> CVICDPSVVLALKSLEKDYLPGHLDAKHHKAMMERVENAVKDFQELSLNEDAYMGVVDEATLQKGSWSLLKDLKRITDSDVKGDLFVKELFWMLHLQKETFATYVARFQKEAYCPNKCGVMLQTLIWCKNCKKEVHACRKSYDCGERNVEVPQMEDMILDCELNWHQASEGL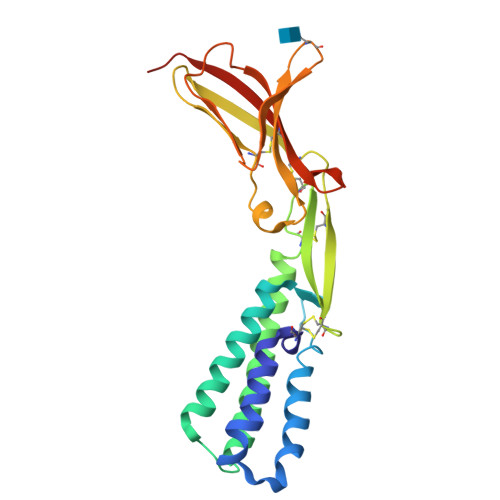TDYSFYRVWGNNTETLVSKGKEATLTKPMVGPEDAGSYRCELGSVNSSPATIINFHVTVLPGRVLPR> MGNNSESKGSASDSKGAETFTYKAENGNVKIPKHPKRVVVMADGYYGYFKTLGINVVGAPENVFKNPYYKGKTNGVENIGDGTSVEKVIDLNPDLIIVWTTQGADIKKLEKIAPTVAVKYD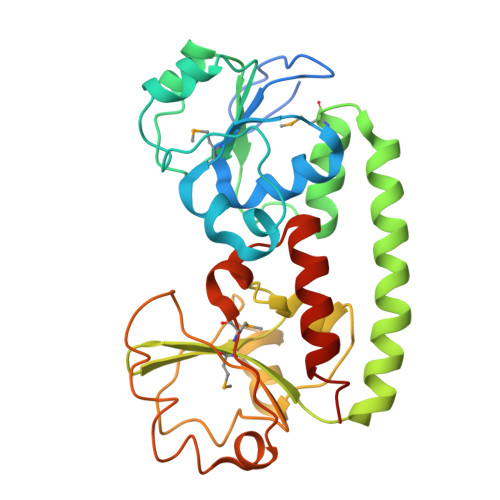KLDNIEQLKEFAKMTGTEDKAEKWLAKWDKKVAAAKTKIKKAVGDKTISIMQTNGKDIYVFGKDFGRGGSIIYKDLGLQATKLTKEKAIDQGPGYTSISLEKLPDFAGDYIFAGPWQSGGDDGGVFESSIWKNLNAVKNGHVYKMDPIGFYFTDPISLEGQLEFITESLTKLEHHHHHH>[2x]GPYMIQEEEWDRDLLLDPAWEKQQRKTFTAWCNSHLRKAGTQIENIEEDFRNGLKLMLLLEVISGERLPKPDRGKMRFHKIANVNKALDYIASKVVKLVSIGAEEIVDGNVKMTLGMIWTIILRFAIQDISVEETSAKEGLLLWCQRKTAPYRNVNIQNFHTSWKDGLGLCALIHRHRPDLIDYSKLNKDDPIGNINLAMEIAEKHLDIPKMLDAEDIVNTPKPDERAIMTYVSCFYHAFAGAEQAETAA

α-Actinin-2 (ACTN2) is the only muscle isoform of α-actinin expressed in cardiac muscle. All four isoforms of α-actinin consist of an N-terminal actin binding domain (ABD) comprising two calponin homology (CH) domains, connected via a flexible linker, which allows for conformational flexibility in the ABDs, to a rod domain. Thus ACTN2 is important in cross-linking actin and titin filaments in the Z-disc. We have investigated the effects of two mutations identified from HCM patients, A119T and G111V, on the secondary and tertiary structure of a purified actin binding domain (ABD) of ACTN2 by circular dichroism and X-ray crystallography, and show small but distinct changes for both mutations.

The original family reported to have an association of the A119T mutation with HCM, had a variable phenotype, with some patients only developing heart failure at the age of 75, and others showing heart failure at ages 36–44. The ABD was in the ‘closed’ conformation in all the structures, as found for other structures of the ABDs for the second striated muscle isoform ACTN3, and the two non-muscle isoforms ACTN1. However, although continuous densities are observed for the loop region at residues 110–120 in both the WT and the A119T mutant structure, this region is disordered for G111V mutant between residues 112 and 117. For both the WT and A119T mutant structure, Val112 is orientated towards the interior of the molecule packing the side chain into a hydrophobic region. G111V lies just outside one of the three stretches of amino acid residues thought to mediate actin binding (residues 41–50, 116–140 and 145–165, reviewed in [31]) and A119T lies within one of these stretches. A119T is within the binding region itself, and its alterations to the structure may be expected to have a small effect on binding. The A119T mutation has an intermediate effect with Tm (60.8°C) only slightly less than WT. The Kd was increased ∼2-fold for the A119T mutant, and ∼1.2-fold for the G111V mutant constructs compared with the WT ABD.> AKKIGLFYGTQTGKTESVAEIIRDEFGNDVVTL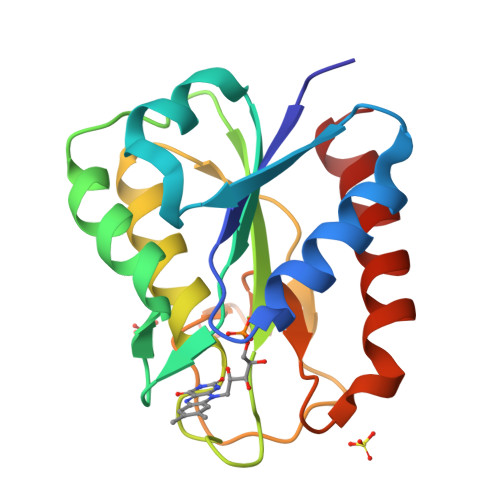HDVSQAEVTDLNDYQYLIIGCPTWNIGELQSDWEGLYSELDDVDFNGKLVAYFGTGDQIGFADNFQDAIGILEEKISQRGGKTVGYWSTDGYDFNDSKALRNGKFVGLALDEDNQSDLTDDRIKSWVAQLKSEFGL Cytosine 5'-[gamma-thio]triphosphate | C9 H16 N3 O13 P3 S | 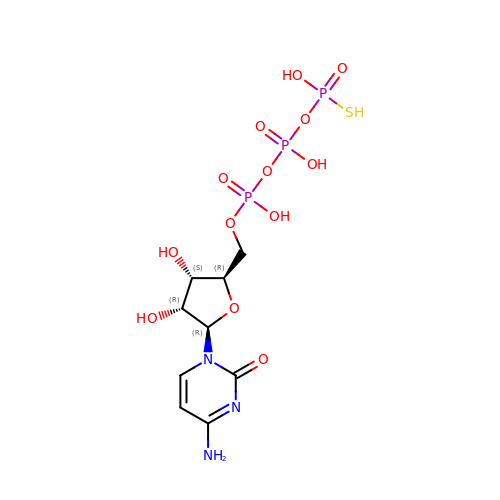BMMOFBYKCSBIJP-XVFCMESISA-N>MSFTTGSTLQHQEAQLQGAKDETVTQLEQRAAGGASHELQSDISKMKTEDDGSFKRKAASFRNWIQPNGDFTPEKGRYHLYVSYACPWATRTLIVRKLKGLEDFIGVTVVSPRMGSNGWPFANVDPFPAADSDPLNNAQHVKDLYLKVKPDYDGRFTVPVLWDKHTGTIVNNESSEIIRMFNTAFNHLLPEDKAKLDLYPESLRAKIDEVNDWVYDTVNNGVYKSGFASTQKAYEAAVIPLFESLDRLEKMLEGQDYLIGGQLTEADIRLFVTIVRFDPVYVTHFKCNLRTIR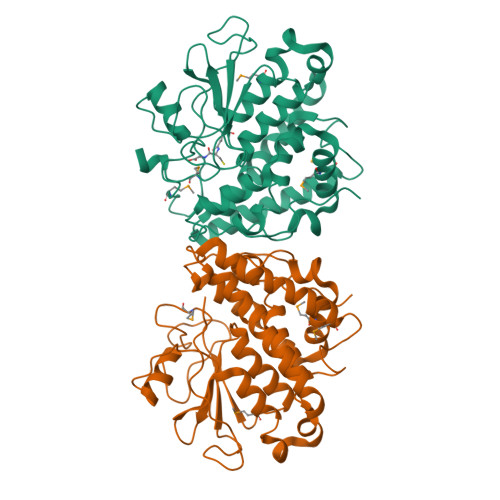DGYPNLHRWMRKLYWGNPAFKDTCNFEHIKTHYFWSHTFINPHRIVPIGPIPDILPLDA[2x]>[2x]MHHHHHHAMEEVTIKANLIFANGSTQTAEFKGTFEKATSEAYAYAD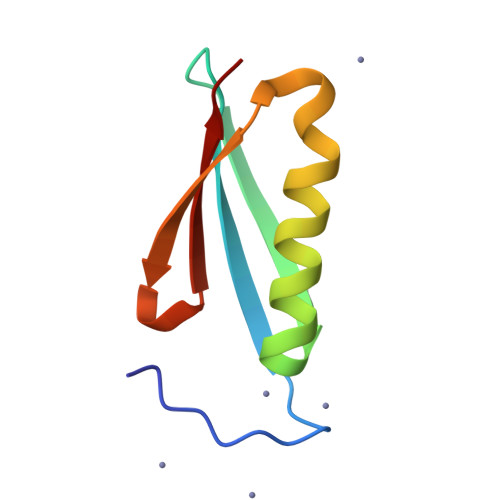TLKKDNGEWTVDVADGGYTLNIKFAG The eukaryotic wobble adenosine-to-inosine modification is catalysed by the ADAT (ADAT2/ADAT3) complex that modifies up to eight tRNAs, requiring a full tRNA for activity. Our structure and associated enzymatic and biophysical analyses reveal that while ADAT2 active site catalyses the deamination reaction, ADAT3 active site is inactivated by the replacement by a valine of the glutamate involved in proton shuttling during catalysis but also by the capping of its zinc-binding pocket and the loss of tRNA recognition determinants. Our results show that the ADAT3 N-terminal domain adopts a fold that shares similarity with the ferredoxin-like domains (FLD) of other tRNA-modifying enzymes, yet with an additional specific structural subdomain, containing V128, which forms a loose interface between ADAT3 N- and C-terminal domains. ADAT3 N-terminal domain is essential for tRNA binding and deamination by ADAT and can rotate with respect to the catalytic domain formed by ADAT2 and the ADAT3 C-terminal domain, without affecting the structure of this latter catalytic domain.

We observe that the equivalent valine 128 in mouse ADAT3 is part of a large hydrophobic core comprising I43, A45, A47, L69, L75, L93, L96, V126, P129 and W146. This hydrophobic core is located in the centre of ADAT3-N and is responsible for the tight interaction between the ADAT3-N FLD and the additional structural subdomain of ADAT3-N. This suggested that the V128M mutation would affect the overall folding of ADAT3-N. To test this hypothesis, we generated constructs bearing the V128M mutation but also the V128L or V128I mutations, those latter two substitutions having potentially a milder effect on ADAT3-N folding. Whereas the crystals with the V128I and V128M mutants, which showed stronger aggregation, did not diffract sufficiently, we were able to collect a full data set at 2.0 Å resolution for the V128L mutant. The structure of the ADAT-V128L complex was refined with good data collection and refinement statistics. The same crystallographic space group and unit cell as well as the similar resolution obtained for both WT and V128L ADAT complexes allowed the precise analysis of the structural changes occurring upon the V128L mutation. Superposition of the complexes showed that both ADAT3-N and the ADAT catalytic domain are mostly unaffected by the mutation. In details, however, we observed that the main chain of residues involved in the V128 central hydrophobic core and of their neighbours is moving away from the core by about 0.3–0.9 Å. We found that these movements are mainly propagated within the ADAT3-N specific structural subdomain but much less in the FLD, which displays a more stable fold due to its tighter packing. A bulkier methionine in place of the leucine at position 128 will have a more substantial effect on the ADAT3-N structure and we expect the movements observed in the case of the V128L mutation to be larger in the V128M mutant.

> MEEKVESTTTPDGPCVVSVQETEKWMEEAMRMAKEALENIEVPVGCLMVYNNEVVGKGRNEVNQTKNATRHAEMVAIDQVLDWCHQHGQSPSTVFEHTVLYVTVEPCIMCAAALRLMKIPLVVYGCQNERFGGCGSVLNIASADLPNTGRPFQCIPGYRAEEAVELLKTFYKQENPNAPKSKVRKKDCQKS;> MEPTSGFAEQPGPVKAESEEQEPAQWQALPVLSEQQSGAVELILAYAAPVLDKRQTSRLLREVSAVYPLPAQPHLKRVRPSRSAGGAQSSDLLLCLAGPSAGPRSLAELLPRPAVDPRGLGTPFLVPLPARPPLTRSQFEEARAHWPTSFHEDKQVTSALAGQLFSTQERAAMQTHMERAVCAAQRAAAQGLRAVGAVVVDPASDRVLATGHDCSSVASPLLHAVMVCIDLVAQGQGEDSLPYVCTGYDLYVTREPCVMCAMALVHARIQRVFYGAPSPDGALGTLFRVHARPDLNHRFQVFRGILEDQCRQLDPDP> MAKIYKDEDISLEPIKNKTIAILGYGSQGRAWALNLRDSGLNVVVGLERQGDSWRRAIDDGFKPMYTKDAVAIADIIVFLVPDMVQKSLWLNSVKDFMKKGADLVFAHGFNIHFKIIEPPKDSDVYMIAPKSPGPIVRRSYEMGGGVPALVAVYQNVSGEALQKALAIAKGIGCARAGVIESTFKEETETDLFGEQVILVGGIMELIKASFETLVEEGYQPEVAYFETVNELKLIVDLIYEKGLTGMLRAVSDTAKYGGITVGKFIIDKSVRDKMKIVLERIRSGEFAREWIKEYERGMPTVFKELSELEGSTIETVGRKL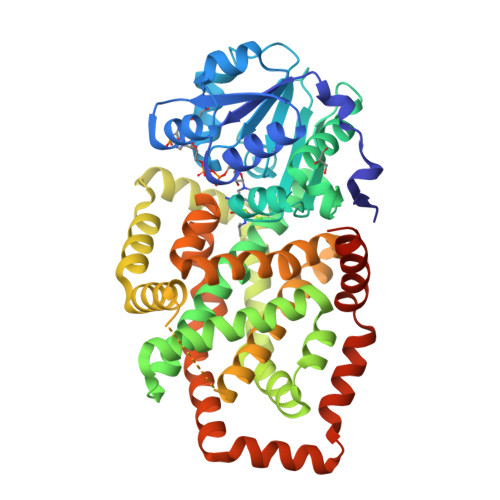REMMFRGMKQISSHETDLFGEQVILVGGIMELIKASFETLVEEGYQPEVAYFETVNELKLIVDLIYEKGLTGMLRAVSDTAKYGGITVGKFIIDKSVRDKMKIVLERIRSGEFAREWIKEYERGMPTVFKELSELEGSTIETVGRKLREMMFRGMKQISSHLEHHHHHH> HHHHHHSSGLVPRGSHMQFVNKQFNYKDPVNGVDIAYIKIPNVGQMQPVKAFKIHNKIWVIPERDTFTNPEEGDLNPPPEAKQVPVSYYDSTYLSTDNEKDNYLKGVTKLFERIYSTDLGRMLLTSIVRGIPFWGGSTIDTELKVIDTNCINVIQPDGSYRS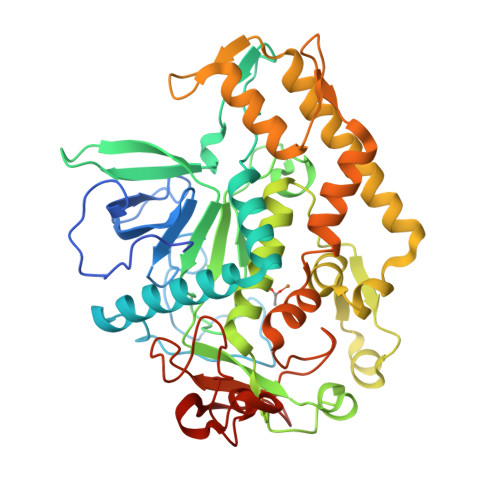EELNLVIIGPSADIIQFECKSFGHEVLNLTRNGYGSTQYIRFSPDFTFGFEESLEVDTNPLLGAGKFATDPAVTLAHELIHAGHRLYGIAINPNRVFKVNTNAYYEMSGLEVSFEELRTFGGHDAKFIDSLQENEFRLYYYNKFKDIASTLNKAKSIVGTTASLQYMKNVFKEKYLLSEDTSGKFSVDKLKFDKLYKMLTEIYTEDNFVKFFKVLNRKTYLNFDKAVFKINIVPKVNYTIYDGFNLRNTNLAANFNGQNTEINNMNFTKLKNFTGLFEF> GPLGSDQTWVQCDACLKWRKLPDGMDQLPE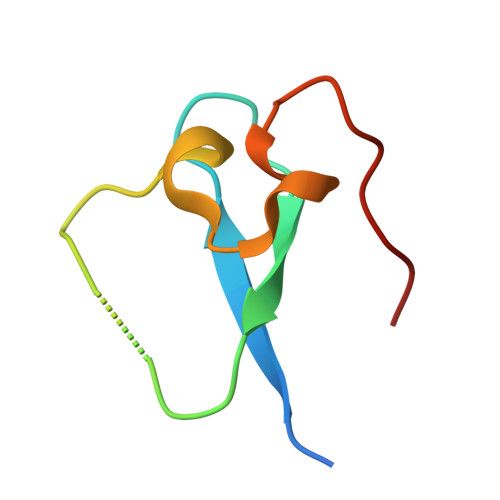KWYCSNNPDPQFRNCEVPEEPED> MVEATAQETDRPRFSFSIAAREGKARTGTIEMKRGVIRTPAFMPVGTAATVKALKPETVRATGADIILGNTYHLMLRPGAERIAKLGGLHSFMGWDRPILTDSGGYQVMSLSSLTKQSEEGVTFKSHLDGSRHMLSPERSIEIQHLLGSDIVMAFDECTPYPATPSRAASSMERSMRWAKRSRDAFDSRKEQAENAALFGIQQGSVFENLRQQSADALAEIG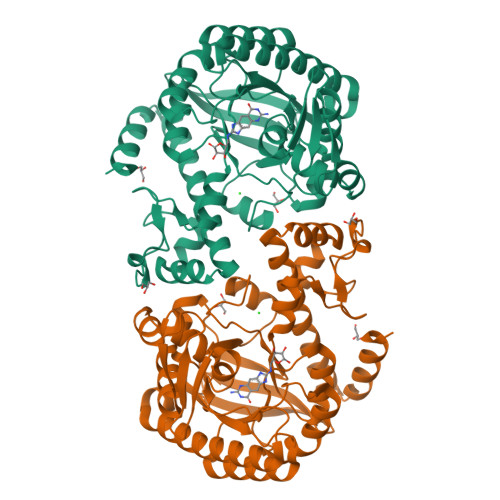FDGYAVGGLAVGEGQDEMFRVLDFSVPMLPDDKPHYLMGVGKPDDIVGAVERGIDMFDCVLPTRSGRNGQAFTWDGPINIRNARFSEDLKPLDSECHCAVCQKWSRAYIHHLIRAGEILGAMLMTEHNIAFYQQLMQKIRDSISEGRFSQFAQDFRARYFARNS> MFIRIKCFSKQPIAKKVSREVSAYLEYTGNNTWEGHISGQGVSNLQTKLIN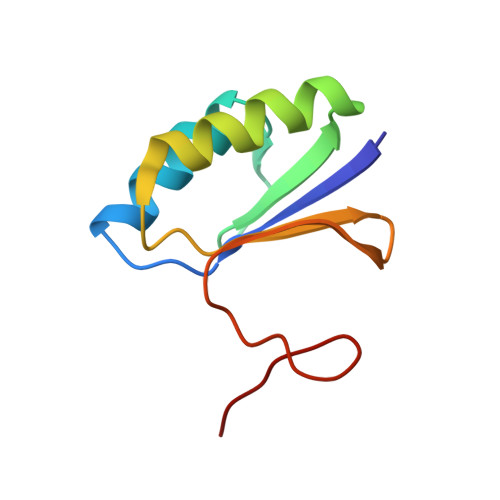VGKGVKVVCNYQDKVLFAIGNVAMSDTGSVPKY> ASTSKTIEELQQEMEDLDADTTITVVQRETQKARIREQIETLRAQQMVRPSEAQLQPDVTPTQIVTFEPPRVTGFGALWIPRQQRNYMTTAYIEKIKAYVPHSNLIESG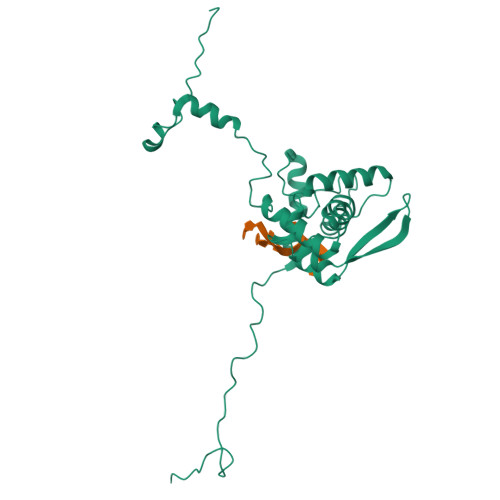LASEAQLTSWIENTCRDYQVSMDVFMTTVLPAWIVNCIINGTSQERTNEHTWRAVIMANMEDQEVLYYPIKPIIVNAQPTLRQVMRHFGEQAVAQYMNSLQAGKPFTVKGAVTAGYANVQDAWLGIDFLRDTMQLTTKQMEVKHQIIAANVTRRKIRVFALAAPGDGDELDTERHVVDDVARGRHSLRGAQLD Cobalamin-dependent methionine synthase (MS) is a key enzyme in methionine and folate one-carbon metabolism. MS is a large multi-domain protein capable of binding and activating three substrates: homocysteine, folate, and S-adenosylmethionine for methylation. Achieving three chemically distinct methylations necessitates significant domain rearrangements to facilitate substrate access to the cobalamin cofactor at the right time. Here, we use a thermophilic MS homolog (tMS) as a functional MS model.

To interrogate the structural basis of cofactor loading, we sought to crystallize the Cap:Cob:Act tridomain in its apo-form, then performed soaking experiments to obtain the holo-Cap:Cob:Act complex. We selected cyanocobalamin (CN-Cbl), a stable and synthetic Cbl that does not support catalysis. To that end, apo-Cap:Cob:Act tMS crystals were soaked with CN-Cbl, yielding a structure of the holo-complex, solved to 2.95 Å resolution and one in the apo-form obtained prior to soaking, solved to 2.4 Å resolution. The apo-Cap:Cob:Act structure aligns well with the respective portion of the apo-tMS full-length structure, with an RMSD of 2.34 Å. The Act domain is positioned over the Cob domain, indicating that the apo-tridomain structure is found in a conformation that has previously been associated with the enzyme entering the reactivation conformation (Act-on, Cap-off). However, the loop containing His761, relevant to reactivation and cofactor loading, displays some marked differences. Structural alignment with the apo-Cap:Cob:Act structure shows that His761 imidazole side chain of the apo-tridomain is ~6 Å from the docked Cbl cofactor/Co, in an orientation facing away from the cofactor. The captured apo structures (tMS full-length and Cap:Cob:Act tridomain) and the tridomain holo-structure highlight the preformed cobalamin pocket, which is solvent-exposed and thus readily accessible even in crystallo. In order for tMS to undergo reactivation, His761 and the helix α1 adjacent loop on which it is found would have to reorient itself to bind cobalamin in the His-on, base-off mode, and Tyr1132 would need to swing and “uncap” the upper axial portion of the cobalamin cofactor. Furthermore, the captured apo-Cap:Cob:Act structure would fulfill the reorganization requirements, priming the cobalamin cofactor for reductive methylation.

>[3x]PLLERLKRRVVEGRKQGLEADLEEALKAGHKPLDLINGPLLAGMKEVGDLFGAGKMQLPFVLQAAEVMKRAVAYLEPHMEKKGEGKGTLVLATVKGDVHDIGKNLVDIILSNNGYRVVNLGIKVPIEEILKAVEAHKPHAVGMSGLLVKSTLVMKENLEYMRDRGYTLPVILGGAALTRSYVEELRAIYPNVYYAEDAFEGLRLMEELTGHAPPELTRKAPARPKREAPKVAPRARPVGEAPAVPRPPFFGVRVEEGLDLATIAHYVNKLALYRGQWGYSRKGLSREAWQALVEREAEPVFQRLLKEAMAEGWLEPKVLYGFFPVAREGEELLVFSPETGEVLERFRFPRQKGGGLSLVDYFRPRFAAPLGDEADWMPKEAFRAGARDVLGVQLVTMGEAPSRKAQALFASGAYQDYLFVHGFSVEMTEALAEYWHKRMRQMWGIAHQDATEIQKLFQQGYQGARYSFGYPACPDLADQAKLDRLMGFHRVGVRLTENFQLEPEHATSALVVHHPEARYFSVD> MRGSHHHHHHGMASMAMYQNMLVVIDPNQDDQPALRRAVYLHQRIGGKIKAFLPIYDFSYEMTTLLSPDERTAMRQGVISQRTAWIREQAKYYLEAGVPIEIKVVWHNRPFEAIIQEVIAGSHDLVLKMAHQADRLEAVIFTPTDWHLLRK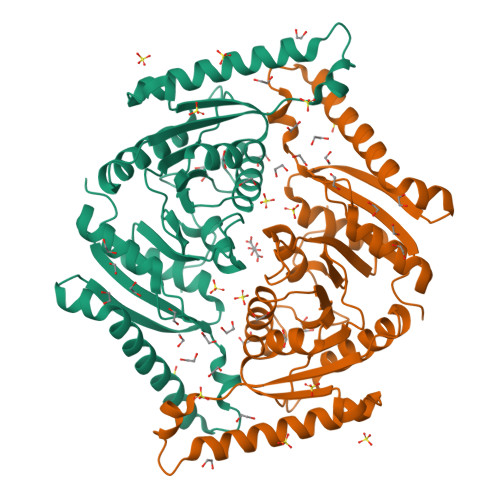CPSPVWMVKDQPWPEGGKALVAVNLASEEPYHNALNEKLVKETLQLAEQVNHTEVHLVGAYPVTPINIAIELPEFDPSVYNDAIRGQHLLAMKALRQKFSIDEKVTHVEKGLPEEVIPDLAEHLQAGIVVLGTVGRTGLSAAFLGNTAEQVIDHLRCDLLVIKPDEYQTPVELDDEDD>EDNSCPPHWKNFTDKCYYFSVEKEIFEDAKLFCEDKSSHLVFINTREEQQWIKKQMVGRESHWIGLTDSERENEWKWLDGTSPDYKNWKAGQPDNWGHGHGPGEDCAGLIYAGQWNDFQCEDVNNFICEKDRETVLSSA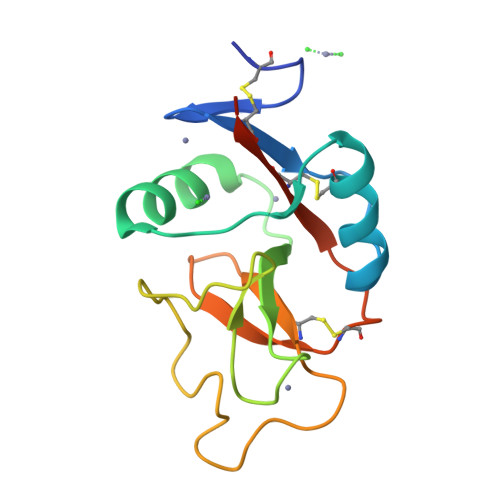L[4x]> GGGRTNVPNGYSQNDIQLMANAVYGESRGE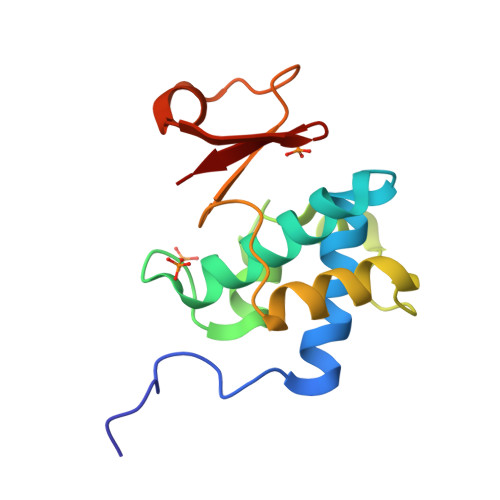PYLGQVAVAAVILNRVTSASFPNTVSGVIFEPRAFTAVADGQIYLTPNETAKKAVLDAINGWDPTGNALYYFNPDTATSKWIWTRPQIKKIGKHIFCK>KKSPSAGSGSNGGNKKISQEEGEDNGGEDNKKLRGALSSAILSEKPNVKWEDVAGLEGAKEALKEAVILPVKFPHLFKGNRKPTSGILLYGPPGTGKSYLAKAVATEANSTFFSVSSSDLVSKWMGESEKLVKQLFAMARENKPSIIFIDQVDALTGTRGEGESEASRRIKTELLVQMNGVGNDSQGVLVLGATNIPWQLDSAIRRRFERRIYIPLPDLAARTTMFEINVGDTPSVLTKEDYRTLGAMTEGYSGSDIAVVVKDALMQPIRKIQSATHFKDVSTEDDETRKLTPSSPGDDGAIEMSWTDIEAD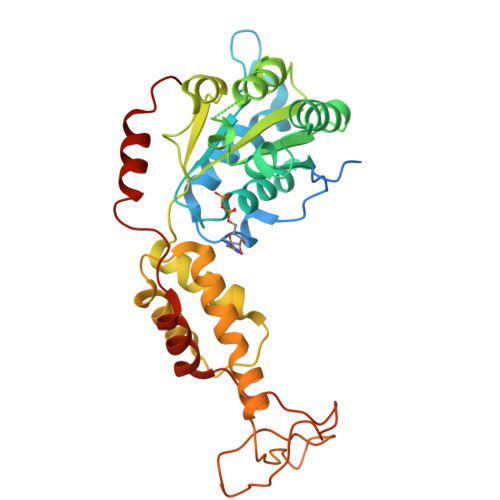ELKEPDLTIKDFLKAIKSTRPTVNEDDLLKQEQFTRDFGQEGN[3x]>[2x]XMEAAHSKSTEECLAYFGVSETTGLTPDQVKRHLEKYGHNELPAEEGKSLWELVIEQFEDLLVRILLLAACISFVLAWFEEGEETITAFVEPFVILLILIANAIVGVWQERNAENAIEALKEYEPEMGKVYRADRKSVQRIKARDIVPGDIVEVAVGDKVPADIRILSIKSTTLRVDQSILTGESVSVIKHTEP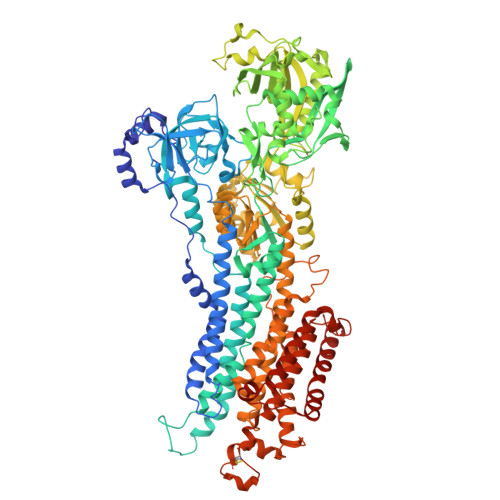VPDPRAVNQDKKNMLFSGTNIAAGKALGIVATTGVSTEIGKIRDQMAATEQDKTPLQQKLDEFGEQLSKVISLICVAVWLINIGHFNDPVHGGSWIRGAIYYFKIAVALAVAAIPEGLPAVITTCLALGTRRMAKKNAIVRSLPSVETLGCTSVICSDKTGTLTTNQMSVCKMFIIDKVDGDFCSLNEFSITGSTYAPEGEVLKNDKPIRSGQFDGLVELATICALCNDSSLDFNETKGVYEKVGEATETALTTLVEKMNVFNTEVRNLSKVERANACNSVIRQLMKKEFTLEFSRDRKSMSVYCSPAKSSRAAVGNKMFVKGAPEGVIDRCNYVRVGTTRVPMTGPVKEKILSVIKEWGTGRDTLRCLALATRDTPPKREEMVLDDSSRFMEYETDLTFVGVVGMLDPPRKEVMGSIQLCRDAGIRVIMITGDNKGTAIAICRRIGIFGENEEVADRAYTGREFDDLPLAEQREACRRACCFARVEPSHKSKIVEYLQSYDEITAMTGDGVNDAPALKKAEIGIAMGSGTAVAKTASEMVLADDNFSTIVAAVEEGRAIYNNMKQFIRYLISSNVGEVVCIFLTAALGLPEALIPVQLLWVNLVTDGLPATALGFNPPDLDIMDRPPRSPKEPLISGWLFFRYMAIGGYVGAATVGAAAWWFMYAEDGPGVTYHQLTHFMQCTEDHPHFEGLDCEIFEAPEPMTMALSVLVTIEMCNALNSLSENQSLMRMPPWVNIWLLGSICLSMSLHFLILYVDPLPMIFKLKALDLTQWLMVLKISLPVIGLDEILKFIARNYLEG(2S,3R)-4-(2-aminoethylcarbamoyloxy)-2-[(2-methanoylindolizin-3-yl)amino]-3-methyl-3-sulfino-butanoic 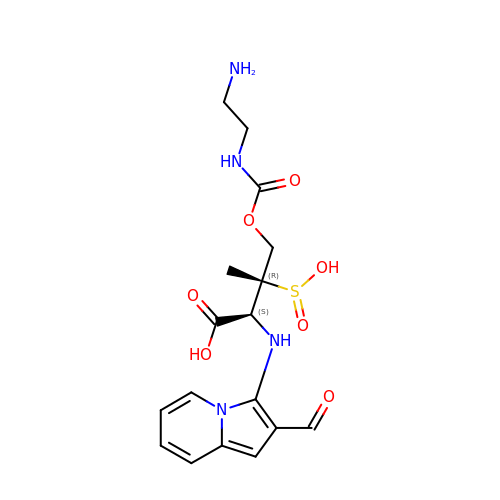acid | C17 H22 N4 O7 S | UGXGYKKZKHIUJW-GUYCJALGSA-N> NQPVNQPILAAAQSLHREATKWSSKGNDIIAAAKRMALLMAEMSRLVRGGSGTKRALIQCAKDIAKASDEVTRLAKEVAKQCTDKRIRTNLLQVCERIPTISTQLKILSTVKATMLGRTNISDEESEQATEMLVHNAQNLMQSVKETVREAEAASIKIRTDAGFTLRWVRKT

At one level this relies on proper links of the actin network to cadherin receptor-mediated cell-cell adherens junctions, to integrin receptor-directed focal adhesions, and to intercalated discs that are required for muscle cell function and that orchestrate coordinated movement. These links are provided in part by vinculin, a highly conserved and structurally dynamic protein that stabilizes adhesions complexes and which binds to actin through the agency of its five-helix bundle tail (Vt) domain. All muscle cell types selectively express an alternatively spliced isoform of vinculin, coined metavinculin, which harbors a 68-residue insert positioned between α-helices H1 and H2 of the Vt domain. Metavinculin is always co-expressed with vinculin in muscle but, unlike vinculin, it cannot homodimerize and rather forms heterodimers with vinculin, an interaction thought important for metavinculin functions. Importantly, although its insert does not bind to actin, metavinculin differs markedly from vinculin in its control of the actin network, where the metavinculin tail (MVt) domain (a surrogate for activated metavinculin) induces a fine meshwork of actin filaments while Vt provokes the formation of tight actin bundles.

To define the molecular underpinnings of metavinculin's unique functions we solved the crystal structures of full-length human metavinculin (124 kDa) and its tail domain to 3.4 Å and 2.2 Å resolution, respectively. Rather, an α-helix of the metavinculin insert (coined H1′) and its amino-terminal extended coil replace the H1 α-helix and its amino-terminal extended coil that are present in Vt, which are no longer part of the MVt domain but are rather disordered in the metavinculin structure. Indeed, the H1′ for H1 replacement in metavinculin results in a new five-helix bundle (that is comprised of α-helices H1′ and H2–H5; residues 959–1,130) that closely mimics the five-helix bundle found in Vt (comprised of α-helices H1–H5; residues 891–1,062), where it can be superimposed with an r.m.s.d. of 0.69 Å (for 153 equivalent Cα positions). Thus, the true helical bundle MVt domain (residues 959–1,134) lacks the H1 α-helix of vinculin. However, a comparison of the tail domain structures of metavinculin with that of vinculin demonstrated that α-helix H1′ has several additional interactions with the four-helix bundle H2–H5 compared to α-helix H1. Specifically, there are two additional hydrophobic and hydrogen bond interactions in metavinculin, and there is also an electrostatic interaction of Arg-1107 with Glu-976 present in α-helix H1′, whereas the corresponding residues in Vt do not interact.2,4,6-tris(iodanyl)-5-(octanoylamino)benzene-1,3-dicarboxylic acid | C16 H18 I3 N O5 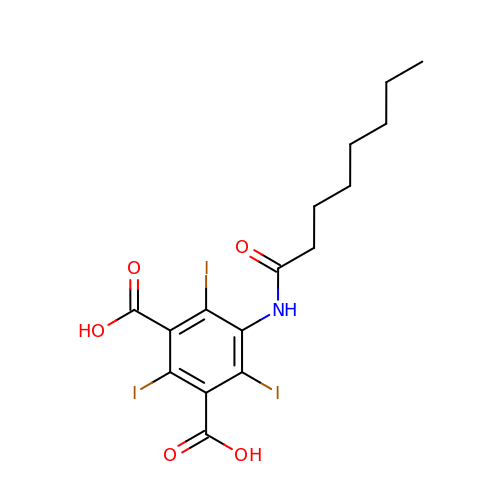| STMIUHPXRYKWPU-UHFFFAOYSA-N> MLTMKDIIRDGHPTLRQKAAELELPLTKE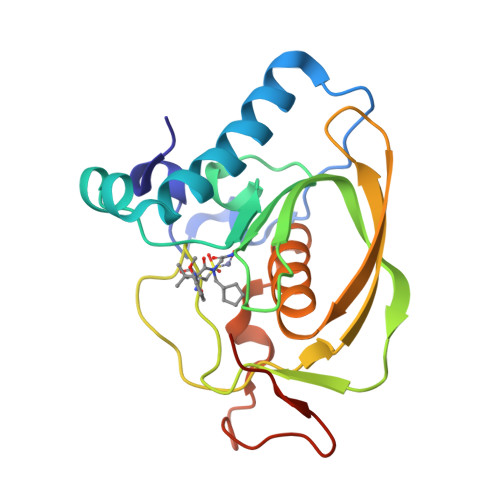EKETLIAMREFLVNSQDEEIAKRYGLRSGVGLAAPQINISKRMIAVLIPDDGSGKSYDYMLVNPKIVSHSVQEAYLPTGEGCLSVDDNVAGLVHRHNRITIKAKDIEGNDIQLRLKGYPAIVFQHEIDHLNGVMFYDHIDKDHPLQPHTDAVEVLEHHHHHH>MVRPSQSMYDRHLTIFSPDGNLYQIEYAIKAVKNTNITSVGVKGENCAVIISQKKMATQYISQDKLLDYNNITNIYNITDEIGCSMVGMPGDCLSMVYKARSEASEFLYSNGYNVNAETLCRNICDKIQVYTQHAYMRLHACSGMIIGIDENNKPELFKFDPSGFCAGYRACVIGNKEQESISVLERLLEKRKKKIQQETIDEDIRNTTILAIEALQTILAFDLKASEIEVAIVSTKNRNFTQISEKEIDNYLTYIAERD[2x];>MADGEYSFSLTTFSPTGKLVQIEYALNRVSSSSPALGIRAKNGVIIATEKKSPNELIEENSIFKIQQISEHIGIVYAGMPGDFRVLLKRARKEAIRYSLQYGSEILVKELVKIIASIVQEFTQTGGVRPFGLSLLICGVDVYGYHLYQIDPSGCYFNWMATCVGKDYQNNMSFLEKRYNKDIEIEDAIHTAILTLKESYEGVLNEKNIEIGVAYDNKPFKILTQNEIKDYLIEIE[2x];>MARRYDSRTTTFSPEGRLYQVEYALEAINNASITIGLITKDGVILGADKVFISKLIDKANNYEKIYKIDKHIFCGVAGLNADANILINQSRLYAQRYLYNYNEVQPVSQLVVQICDIKQSYTQYGGLRPYGVSFLIGGYDTKDGYQLYHTDPSGNYSGWFATAIGTNNLTASSVLKQEWKNDMTLEEGLLLALKTLAKSTDTEIPKSEKIELAYLTNKDGEVYQKYLTEKEIEELIKLYTQK[2x];>MSYDRAITVFSPDGHLLQVEHALEAVKKGGCAVAIKSSNFAVLAVEKKNIPKLQNPKTTEKLIKLDEHNCLAFAGLNADARVLVNKTRLECQRYYLNMDEPAPVDYIAKYVAKVQQKFTHRGGVRPFGIATLIAGFKNNKEICIYQTEPSGIYAAWKAQAIGKNAKIVQEFLEKNYQENMEQKDCIFLALKAIFEVVELSSKNVEVALLTEKDLTFIEEQEINSMVELIDQERTKNNEQNE[2x];>[2x]MFSTRSEYDRGVNTFSPEGRLFQVEYALGAIKLGSTAVGICVNDGVILASERRISSTLIEKDSVEKLLSIDDHIGCAMSGLMADARTLIDYARVECNHYKFIYNENINIKSCVELISELALDFSNLSDSKRKKIMSRPFGVALLIGGVDKNGPCLWYTEPSGTNTRFSAASIGSAQEGAELLLQENYKKDMTFEQAEILALTVLRQVMEDKLSTSNVEICAIKKSDQTFYKYNTDDISRIIDVLPSPVYPTIDMTA;>[2x]MYRNLYDTDNIIYSPEGRLYQVEYASEAIKQGTCAVAIKSKDYVVVSGLKKCISKLSFPQEKIFKIDDYIGISMSGITSDAKVLTKFMQNECLSHKFLYNENINIESLVRSVADKYQKNTQKSSKRAFGVGLMIAAYHNEPCIFETRPNGSYFEYDALSFGARSHASKTYLEKNLHLFEECSLEELILHCLKALKCSLSSESELTISNTALAVVGKNHPWQEISSLQLEEYLSKVKMDAEQEQVEENVQNEANE;>MAGLSAGYDLSVSTFSPDGRLYQVEYIYKSINNNNTALCLECKDGIICCCINSNMDKNKMIKKNSYNRIYHVNNNIIITYSGFDGDARNIIDRARSEANTYYYNFHTNIPLHILVNRISLYIHAYTLYWHMRPFAASIIISSFNEKDKGDIYCIEPNGACYKYSGIVIGKNKEMFKTEIEKKDYKDINVRDAIEDIYKFILTSDDHMNKNNLQNLVNFSWICKESSYEFQNIHEEILTPALNKAVEYIEKLN[2x];>[2x]TTIIGIIYDNGVMLACDSRTSSGTFISNKCSRKINRINENLYVCRSGASAHSQKIIEIIKHYCVSMKNENRKKGRFHEGETIYDETTYDEEIDIDSINYLDYNNNNDNNLVTKNKYFYEDKFNDYNPLVENVAHITKKIIYTNNNFLSCALIFGGYDKIKKQQLYAVNLNGSIIEKHDFAVSGSGSIYIQSYLQDKYKKFMTKKECFNLILNCVKYAMHNDNSSGGLIRIVNITKSFVEEFTVVNTQMNFQY;>TTICGLVCQNAVILGADTRATEGPIVADKNCSKLHYISKNIWCAGAGVAGDLEHTTLWLQHNVELHRLNTNTQPRVSMCVSRLTQELFKYQGYKVCAIVLGGVDVNGPQLYGIHPHGSSCLLPFTALGSGSLNAMAVLEAKYRDNMTIEEGKNLVCEAICAGIFNDLGSGGNVDICVITKDSYQHIRPYKEPNMRLYHLPHPTIYPKGTTPILSEKIEYIKKFISVEDA[2x];>MGSIYNYNGGCVLGMSGSNCVAIACDLRLGANTFTTVSTKFSKIFKMNNNVYVGLSGLATDIQTLYEILRYRVNLYEVRQDAEMDVECFANMLSSILYSNRFSPYFVNPIVVGFKLKHYVDEEGEKKVNYEPYLTAYDLIGAKCETRDFVVNGVTSEQLFGMCESLYVKDQDENGLFET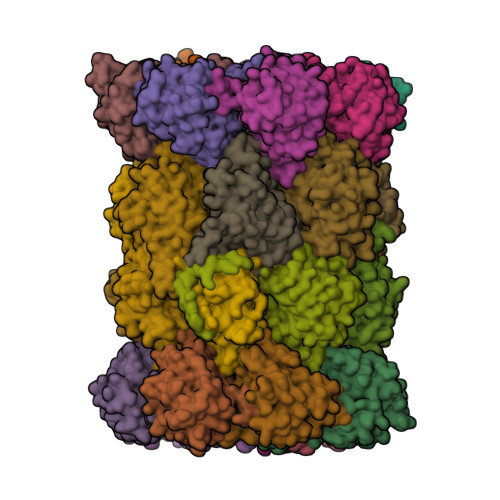ISQCLLSALDRDCISGWGAEVLVLTPEKIIKKKLKARMD[2x];>MDTLIGLRGNNFVVLAADTYSINSIIKLKNDDNTKFYDIHGNKCLLLGGSIGDRLQFGEFIRKNVHLYQYQNNTDMFVKSFAFFTRKNLAYYLRRNPFEVNCLIAGYDKKDGYQLYWCDYLSNMDSVNKGAHGYGAYLVSAILDKYYHENLTVDEALDIFKLCFEELKKRFLLTQINYELRIMYDNKVETQYVTV[2x];>[2x]TTTLAFKFKDGIIVAVDSRASMGSFISSQNVEKIIEINKNILGTMAGGAADCLYWEKYLGKIIKIYELRNNEKISVRAASTILSNILYQYKGYGLCCGIILSGYDHTGFNMFYVDDSGKKVEGNLFSCGSGSTYAYSILDSAYDYNLNLDQAVELARNAIYHATFRDGGSGGKVRVFHIHKNGYDKIIEGEDVFDLHYHYTNPEQKDQYVM;>[2x]MDLILYNDNLTEKKTEKENVIEHGRGFKRWYPYIDNGGTVIGLTGKDYVILAADTRLSLSYSIYTRFCPKISKLTDKCIIGSSGMQSDIKTLHSLLQKKIQLFVLEHSHYPDIHVIARLLCVILYSRRFFPYYAFNILAGVDENNKGVLYNYDSVGSYCEATHSCVGSGSQLILPILDNRVEQKNQLIKNTNFNLGDDINFVKDAITSATERDIYTGDKTLIYVIDKMGINVNTLDLKQD;>[2x]MTLGPVVTGTSVIAIKYKHGIMIAADRKASYGSYAKFQNVERIFKINNKTVMGFSGELADAQYLHELLTRKNINNLSEKKRKEDMYTPQHYHSYVSRVFYVRKNRIDPLFNNIIIAGINSQKYDNNDDNVLLYTNKNNDDEQNEYKNNEEYKEIHKDDLYIGFVDMHGTNFCDDYITTGYARYFALTLLRDHYKDNMTEEEARILINECLRILYFRDATSSNFIQIVKVTSKGVEYEEPYILPCVLNSADYVYPSTLLPPAGCMWGSGSENLYFQGHHHHHHHH> MAHHHHHHMEHNYFYKNSATLKNKHGIKNPRKLYERCAHETAREAVNFRLEPPPGKFDAAYLRTIHWCLFHKTFEWAGVTRDQPFTFEDGSTACM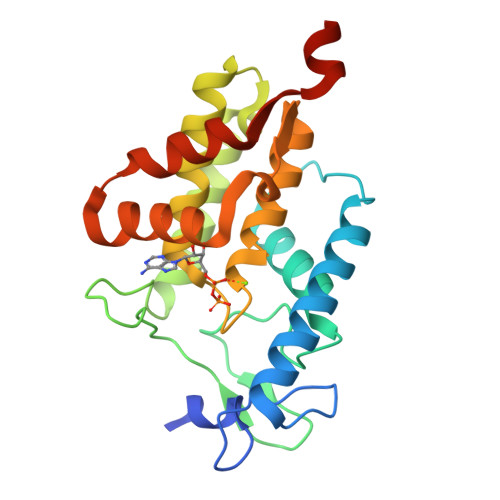PAMRPKGYKVPFAVGSQIQRELKKLEQRLTAKNNLQGLSRQEFAANAAEVFTALDHAHPFRKGNGRTQRMFMEKLGQAAGYKIDFSLITKERMTYASIEAMQHNNPEPMKDLFEDITHPQKSLLLKEFISQM> EQECEPGQTK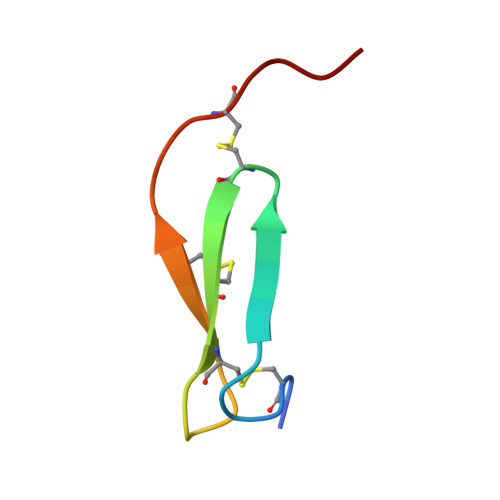KQDCNTCRCGSDGVWACTRMGCPPHA5'-O-[(R)-[(N-acetyl-L-alpha-aspartyl)amino](3-aminopropoxy)phosphoryl]adenosine | C19 H29 N8 O10 P | 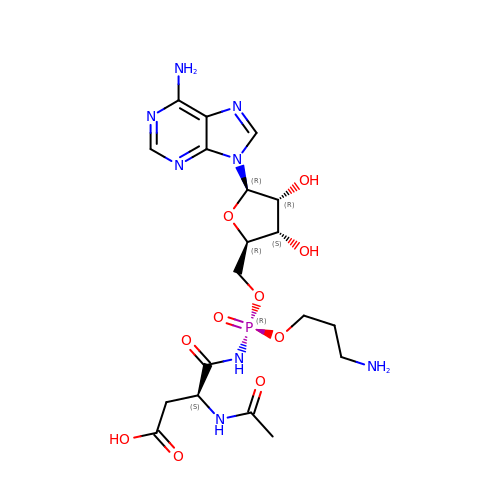VQAWDXQIQSFFEO-HRINIYQMSA-N> ADLGHQTLGSNDGWGAYSTGTTGGSKASSSNVYTVSNRNQLVSALGKETNTTPKIIYIKGTIDMNVDDNLKPLGLNDYKDPEYDLDKYLKAYDPSTWGKKEPSGTQEEARARSQKNQKARVMVDIPANTTIVGSGTNAKVVGGNFQIKSDNVIIRNIEFQDAYDYFPQWDPTAGSSGNWASQY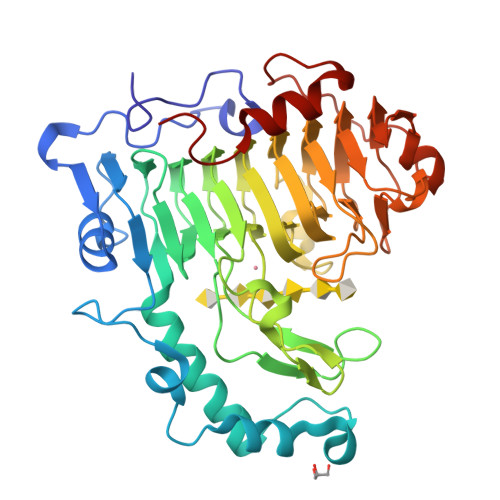DNITINGGTHIWIDHCTFNDGSRPDSTSPKYYGRKYQHHDGQTDASNGANYITMSYNYYHDHDASSIFGSSDSKTSDDGKLKITLHHNRYKNIVQRAPRVRFGQVHVYNNYYEGSTSSSSYPFSYAWGIGKSSKIYAQNNVIDVPGLSAAKTISVFSGGTALYDSGTLLNGTQINASAANGLSSSVGWTPSLHGSIDASANVKSNVINQAGAGKLN>MKIGIIGAMQQEVAILKDLIEDVQEVNQAGCTFYSGQIQGVDVVLLQSGIGKVSAALGTALLISQYAPDVVINTGSAGGFDASLNVGDVVISSEVRHHDADVTAFGYEIGQMAGQPAAFKADEKLMTVAEQALAQLPNTHAVRGLICTGDAFVCTAERQQFIRQHF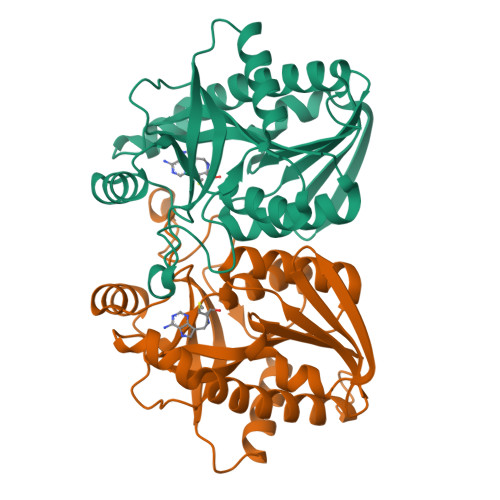PSVVAVEMEASAIAQTCHQFKVPFVVVRAISDVADKESPLSFEEFLPLAAKSSSAMVLKMVELLKENLYFQGHHHHHH[2x]> ARPCIPKSFGYSSVVCVCNATYCDSFDPPTFPALGTFSRYESTRSGRRMELSMGPIQANHTGTGLLLTLQPEQKFQKVKGFGGAMTDAAALNILALSPPAQNLLLK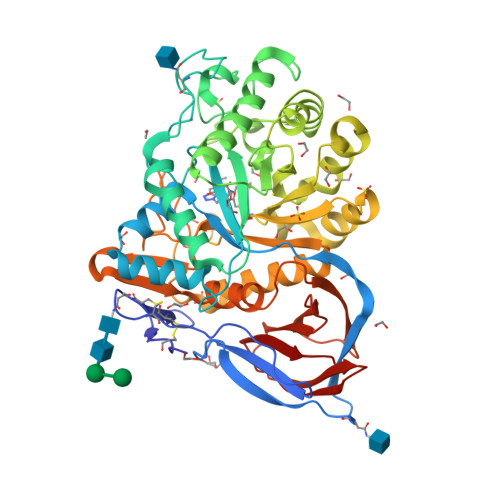SYFSEEGIGYNIIRVPMASCDFSIRTYTYADTPDDFQLHNFSLPEEDTKLKIPLIHRALQLAQRPVSLLASPWTSPTWLKTNGAVNGKGSLKGQPGDIYHQTWARYFVKFLDAYAEHKLQFWAVTAENEPSAGLLSGYPFQCLGFTPEHQRDFIARDLGPTLANSTHHNVRLLMLDDQRLLLPHWAKVVLTDPEAAKYVHGIAVHWYLDFLAPAKATLGETHRLFPNTMLFASEACVGSKFWEQSVRLGSWDRGMQYSHSIITNLLYHVVGWTDWNLALNPEGGPNWVRNFVDSPIIVDITKDTFYKQPMFYHLGHFSKFIPEGSQRVGLVASQKNDLDAVALMHPDGSAVVVVLNRSSKDVPLTIKDPAVGFLETISPGYSIHTYLWRRQ> GAMDNQRQY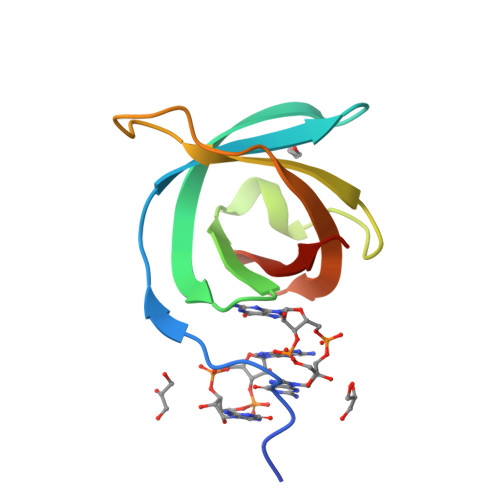PRTPLKCRIRISHPLFGELMAQTRDLSDTGVYVKHPDLTQLPTGSVVTGQVQDLPIDAPILQMEVVRVDAEGVGLRFLSEA> MEAAAGRSSHLGPAPAGRPPRCPLLLQLQLLLLLLLLPPGWVPGAAGTQGAEFPELCSYTWEAVDTKNNMLYKINICGNMGVAQCGPSSAVCMHDLKTDSFHSVGDSLLKTASRSLLEFNTTVNCKQQNHKIQSSITFLCGKTLGTPEFVTATDCVHYFEWRTTAACKKNIFKANKEVPCYAFDRELKKHDLNPLIKTSGAYLVDDSDPDTSLFINVCRDIEVLRASSPQVRVCPTGAAACLVRGDRAFDVGRPQEGLKLVSNDRLVLSYVKEGAGQPDFCDGHSPAVTITFVCPSERREGTIPKLTAKSNCRFEIEWVTEYACHRDYLESRSCSLSSAQHDVAVDLQPLSRVEASDSLFYTSEADEYTYYLSICGGSQAPICNKKDAAVCQVKKADSTQVKVAGRPQNLTLRYSDGDLTLIYFGGEECSSG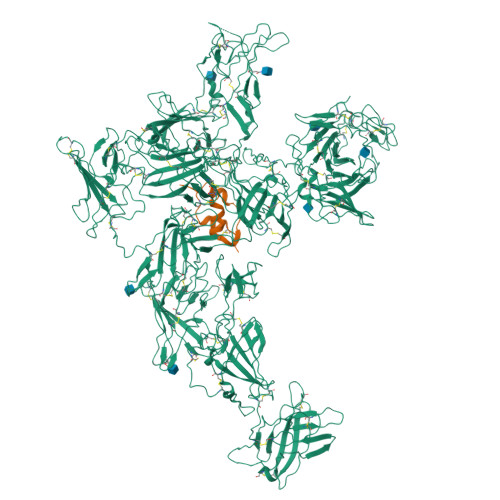FQRMSVINFECNQTAGNNGRGAPVFTGEVDCTYFFTWDTKYACVHEKEALLCGVSDGKQRFDLSALARHSELEQNWEAVDGSQREAEKKHFFINICHRVLQTGQARGCPEDAAVCAVDKNGSKNLGRFISSPTREKGNIQLSYSDGDECGGGQKIITNITLMCKPGDLESAPVLTTSRADGCFYEFEWRTAAACVLSRTEGDNCTVFDSQAGFSFDLTPLTKKDAYKVETDKYEFHINVCGPVSVGACPPDSGACQVSRSDRKSWNLGRSNAKLSYYDGMIQLTYRDGTPYNNEKRTPRATLITFLCDRDAGVGFPEYQEEDNSTYNFRWYTSYACPEEPLECIVTDPVTLDQYDLSRLAKSEGGPGGNWYSLDNGGARSTWRKYYINVCRPLNPVPGCDRYASACQMKYQGEQGSYSETVSISNLGVAKTGPMVEDSGSLLLEYVNGSACTTSDQRRTTYTTRIHLVCSTGSLYTHPIFSLNWECVVSFLWNTAAACPIRITTDIDQVCSIKDPNSGYVFDLNPLNNSRGYVVLGIGKTFLFNVCGDMPACGTLDGKPASGCEAEVQMDDMKTLKPGRLVGLEKSLQLSTEGFITLNYTGLPSHPNGRADAFIIRFVCNDDVYPGTPKFLHQDIDSSLGIRDTFFEFETALACVPSPVDCQVTDPAGNEYDLSGLSKARKPWTAVDTFDEGKKRTFYLSVCTPLPYIPGCHGTAVGCCLVTEDSKLNLGVVQISPQVGANGSLSLVYVNGDKCKNQRFSTRINLECAHTTGSPTFQLQNDCEYVFLWRTVEACPVVRAEGDYCEVRDPRHGNLYNLIPLGLNDTVVRAGEYTYYFRVCGELTSGVCPTSDKSKVISSCQEKRGPQGFQKVAGLFNQKLTYENGVLKMNYTGGDTCHKVYQRSTTIFFYCDRSTQAPVFLQETSDCSYLFEWRTQYACPPYDLTECSFKNEAGETYDLSSLSRYSDNWEAVTGTGSTEHYLINVCKSLSPQAGSDPCPPEAAVCLLGGPKPVNLGRVRDSPQWSQGLTLLKYVDGDLCPDQIRKKSTTIRFTCSESHVNSRPMFISAVEDCEYTFSWPTAAACAVKSNVHDDCQVTNPATGHLFDLSSLSGRAGFTAAYSEKGLVYLSVCGDNENCANGVGACFGQTRISVGKASKRLTYVDQVLQLVYEGGSPCPSKTGLSYKSVISFVCRPEVGPTNRPMLISLDKRTCTLFFSWHTPLACEQTTECSVRNGSSLIDLSPLIHRTGGYEAYDESEDDGSDTSPDFYINICQPLNPMHGLACPAGTAVCKVPVDGPPIDIGRVAGPPILNPIANEVYLNFESSTPCLADRHFNYTSLITFHCKRGVSMGTPKLLRTSVCDFVFEWETPLVCPDEVKTDGCSLTDEQLYYSFNLSSLSKSTFKVTRGPHTYSVGVCTAAAGLDEGGCKDGAVCLLSGSKGASFGRLASMKLDYRHQDEAVILSYANGDTCPPETEDGEPCVFPFVFNGKSYEECVVESRARLWCATTANYDRDHEWGFCKHSTSHRTSVIIFKCDEDADVGRPQVFSEVRGCEVTFEWKTKVVCPPKKMECKFVQKHRTYDLRLLSSLTGSWSFVHNGASYYINLCQKIYKGPQDCSERASVCKKSTSGEVQVLGLVHTQKLDVVDDRVIVTYSKGHYCGDNKTASAVIELTCAKTVGRPSFTRFDVDSCTYHFSWDSRAACAVKPQEVQMVNGTITNPANGRSFSLGDIYFKRFSASGDVRTNGDRYIYEIQLSSITGSSSPACSGASICQRKANDQHFSRKVGTSNQTRYYVQDGDLDVVFTSSSKCGKDKTKSVSSTIFFHCDPLVKDGIPEFSHETADCQYLFSWHTSAVCPLGAGFDEEIAGDDAQEHKGLSERSQAVGAVLSLLLVALTACLLTLLLYKKERREMVMSRLTNCCRRSANVSYKYSKVNKEEEADENETEWLMEEIQPPAPRPGKEGQENGHVAAKSVRAADTLSALHGDEQDSEDEVLTLPEVKVRPPGRAPGAEGGPPLRPLPRKAPPPLRADDRVGLVRGEPARRGRPRAAATPISTFHDDSDEDLLHV;> MAYRPSETLCGGELVDTLQFVCGDRGFYFSRPASRVSRRSRGIVEECCFRSCDLALLETYCATPAKSE> MKYPLVPLVSDLTLSFLVFWLCLPVALLLFLTIVWLHFLLSQESKEDDSDLCFNWEPWSKRPSECGCEETFPGEE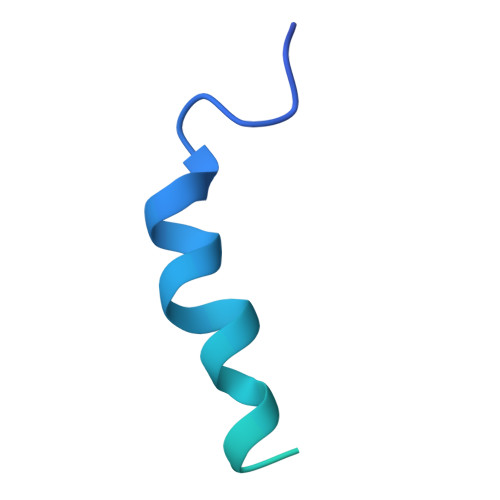DGLHWGGSGSGDYKDDDDK>[2x]MTLVKIGPWGGNGGSAQDISVPPKKLLGVTIYSSD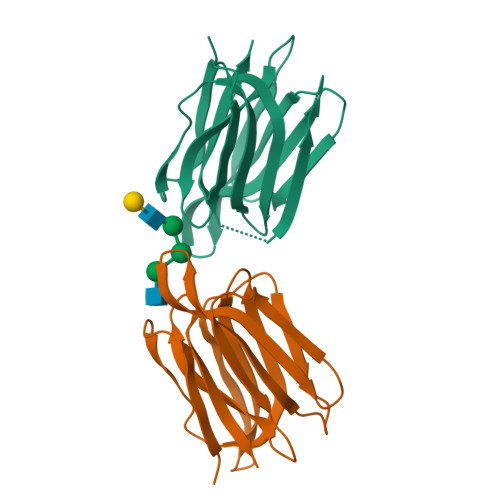AIRSIAFNYIGVDGQEYAIGPWGGGESTSTEIKLGSSEQIKEISGTHGPVYDLADIVTYLKIVTSANNTYEAGVPNGKEFSIPLQDSGHVVGFFGRSGTLIDAIGIYVHP> MDSNTVSSFQVDCFLWHVRKRFADQELGDAPFLDRLRADQASLRGRGSTLGLDIETATRAGKQIVERILEEESDEALKMTIASVPASRYLTDMTLEEMSRDWFMLMPKQKVAGSLCIRMDQAIMDKNIILKANFSVIFDRLETLILLRAFTEEGAIVGEISPLPSLPGHTDEDVKNAIGVLIGGLEWNDNTVRVSETLQRFAWRSSNEDGRPPLPPNQKRKMARTIE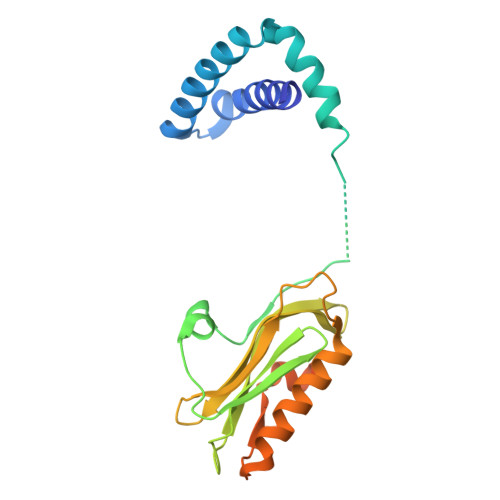SEV>[6x]TLSRDWLAEVRKVLEVRQA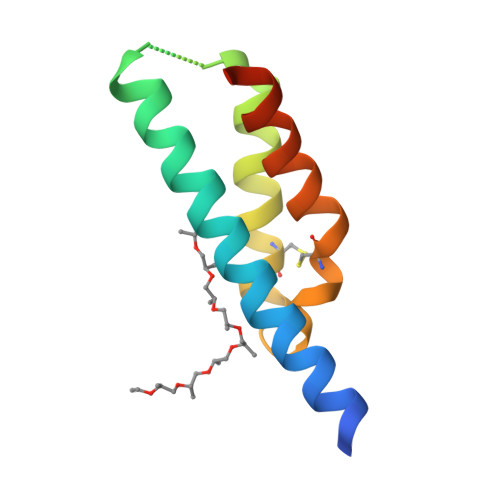LEVIQAEARLQSLRLEGSGSRPLPESVEKARSEVVRCLREHDRRPLNCWQEVEAFKEEVRKLEKGWVDK> MRRCAACLTSLPVSSPTGAAVGAPAAPLKTQAPSNRSLLGYPLRRAAAMEMLYGGICIQHLAQPPFPLRKIQSESLPPPSLQGERDDLELEVKDSTGNVMGYRLFPVNIGI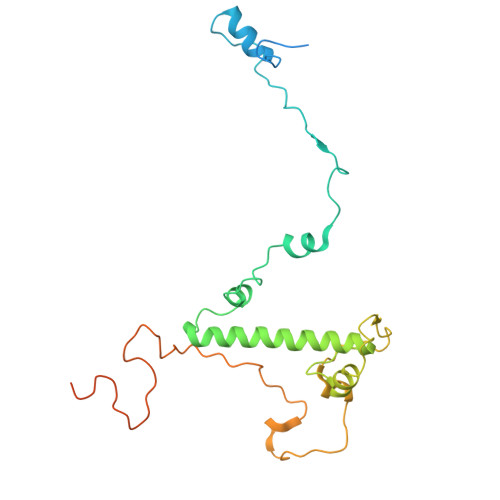RARTESVRVRSEDCYKRFLAQKHCAAAGVPLQFPAPSSITNSNCLATPRAASHFHPPSSSLSLFTRPADSQGGDVGRTTPADVAAYHPRAWRPYQMLKPMPHNWGPAVRSSGVRGPHMQLLQERIDKKGFGWKRKSRSLWQQDISTAGFRPKRYF>EARLEEAVNRWVLKFYFHEALRAFRGSRYGDFRQIRDIMQALLVRPLGKEHTVSRLLRVMQCLSRIEEGENLDCSFDMEAELTPLESAINVLEMIKTEFTLTEAVVESSRKLVKEAAVIICIKNKEFEKASKILKKHMSKDPTTQKLRNDLLNIIREKNLAHPVIQNFSYETFQQKMLRFLESHLDDAEPYLLTMAKKAL[2x];>SRGLE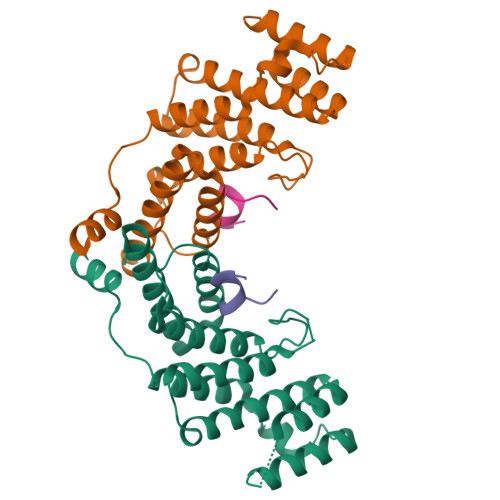VSHRLAPW[2x]>MTEAAAQPHALPADAPDIAPERDLLSKFDGLIAERQKLLDSGVTEPFAIVMEQVKSPTEAVIRGKDTILLGTYNYMGMTFDPDVIAAGKEALEKFGSGTNGSRMLNGTFHDHMEVEQALRDFYGTTGAIVFSTGYMANLGIISTLAGKGEYVILDADSHASIYDGCQQGNAEIVRFRHNSVEDLDKRLGRLPKEPAKLVVLEGVYSMLGDIAPLKEMVAVAKKHGAMVLVDEAHSMGFFGPNGRGVYEAQGLEGQIDFVVGTFSKSVGTVGGFVVSNHPKFEAVRLA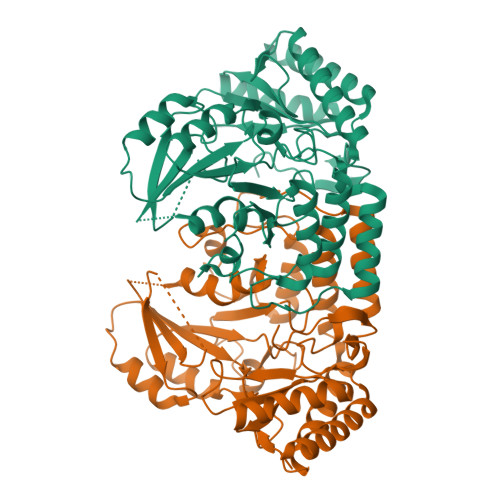CRPYIFTASLPPSVVATATTSIRKLMTAHEKRERLWSNARALHGGLKAMGFRLGTETCDSAIVAVMLEDQEQAAMMWQALLDGGLYVNMARPPATPAGTFLLRCSICAEHTPAQIQTVLGMFQAAGRAVGVIGLE[2x]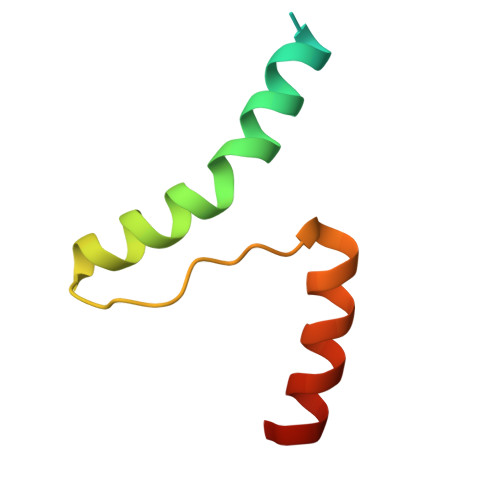> MAYPYDVPDYAAAVKKLTDKQKSRLWELQRNRNFQASRRLGGVEMPLVTLTAAEALARLEELRSHYER> MAHHHHHHMKKILLVGAGDSGKSTIFKQMRLIYNNGFTTEEKTKIKPMIYENILRNMMVLIQATKSLNLPISTEENRQRAEKIEGLEQKILLTTDKVWDSNLAQDIAELWKEPAILQAMARRNEFQIEDSASYYFDNLDRIGKDDYMPSEEDVVRARIKTTGLIEQPFTFKNLPFCMIDVGGQRTERKKWIHHFQGVDSILFVCSLSEFDQKCYEDDSTNRMKESLSLFGDYINSKWFADTLVYLLLNKHDLFVSKIKNGSRLADTFEEYKGPENDPDAAKEFIKDMYKEKDTENRLRDVFFVTALDKANLKERLEQITS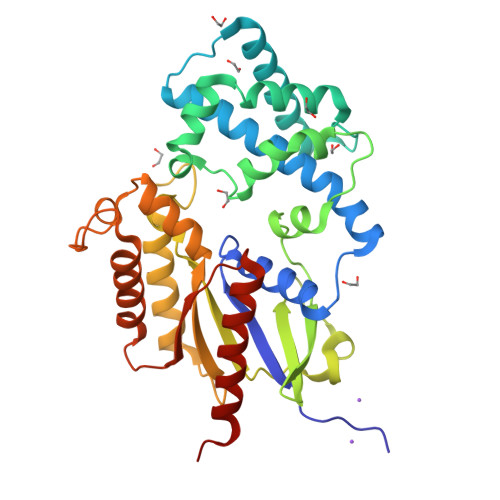DILSAENDL> GSEKCFEPQLLRFFHKNEIWYRTEQAAVARCQCKGPDAHCQRLASQACRTNP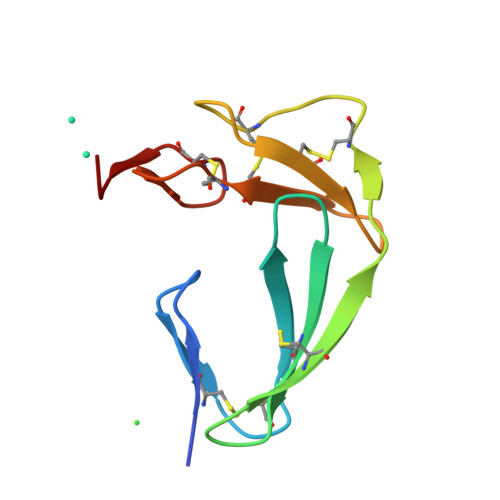CLHGGRCLEVEGHRLCHCPVGYTGPFCDVDTAA> MGNFIITERKKAKEERSNPQTDSMDDLLIRRLTDRNDKEAHLNEL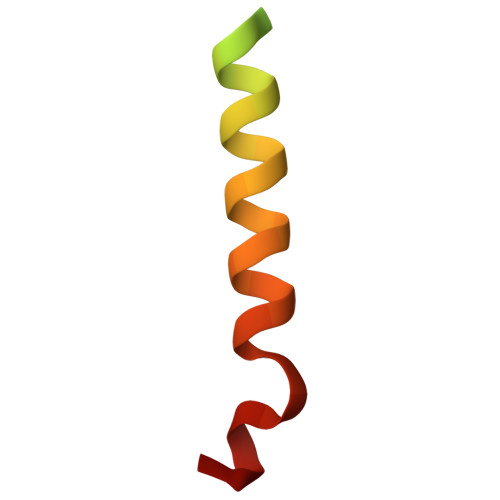F>MVKITRLTTYRLPPRWMFLKVETDEGVTGWGEPVIEGRARTVEAAVHELSDYLIGQDPSRINDLWQTMYRAGFYRGGPILMSAIAGIDQALWDIKGKVLGVPVYELLGGLVRDKMRTYSWVGGDRPADVIAGMKALQAGGFDHFKLNGCEEMGIIDTSRAVDAAVARVAEIRSAFGNTVEFGLDFHGRVSAPMAKVLIKELEPYRPLFIEEPVLAEQAETYA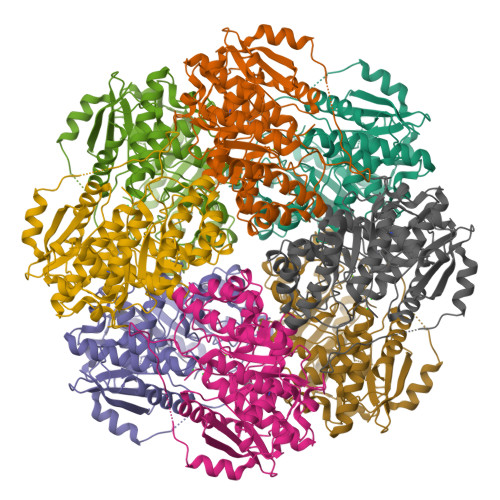RLAAHTHLPIAAGERMFSRFDFKRVLEAGGVSILQPDLSHAGGITECVKIAAMAEAYDVALAPHCPLGPIALAACLHVDFVSWNATLQEQSMGIHYNKGAELLDYVRNKADFALEGGYIRPPRLPGLGVDIDEALVIERSKEAPDWRNPVWRHADGSVAEWAENLYFQSHHHHHHWSHPQFEK[2x]>SMEFQAALSRKVAELVHFLLLKYRAREPVTKAEMLGSVVGNWQYFFPVIFSKASSSLQLVFGIELMEVDPIGHLYIFATCLGLSYDGLLGDNQIMPKAGLLIIVLAIIAREGDCAPEEKIWEELSVLEVFEGREDSILGDPKKLLTQHFVQENYLEYRQVPGSDPACYEFLWGPRALVETSYVKVLHHMVKISGGPHISYPPLHEWVLR[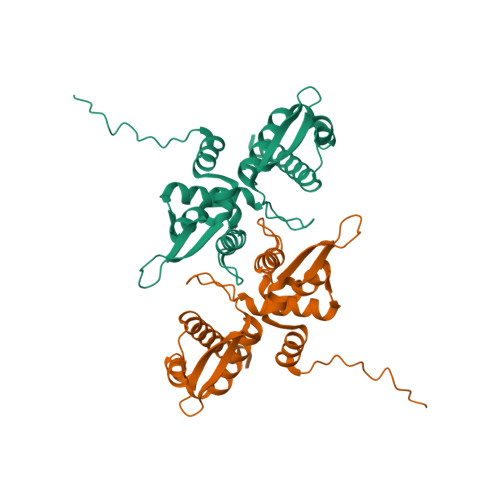3x]>[2x]ETGAAAGDKLLSVCMNSKRHKQEPGPEDELYQECRPWEDNACCTRSTSWEAHLEEPLLFNFSMMHCGLLTPACRKH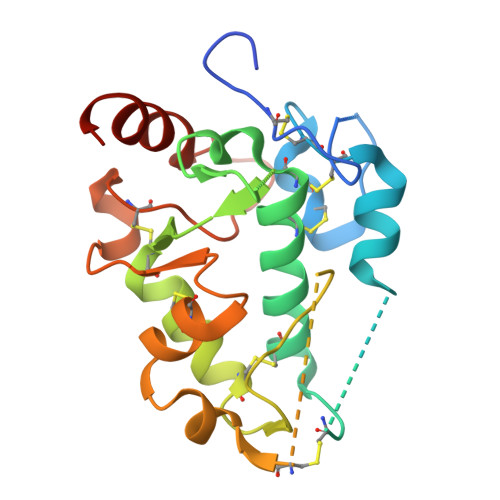FIQAICFHECSPNLGPWIQPVVPNGQEEQRVWGVPLCQEDCEDWWRACHSSLTCKSNWLHGWDWSEEKKHCPAHEPCLPFSYHFPTPDDLCEKIWNNTFKASPERRNSGRCLQKWFEPTLSNPNVEVALHFAHHHHHHHH>[2x]SNAMLVKLAVLFSGNGSNLENILEKLHKKTIGENTYEIVLCLCNKKDAFGIQRAKKFGLNTVIIDHKAYNTREEFDTIL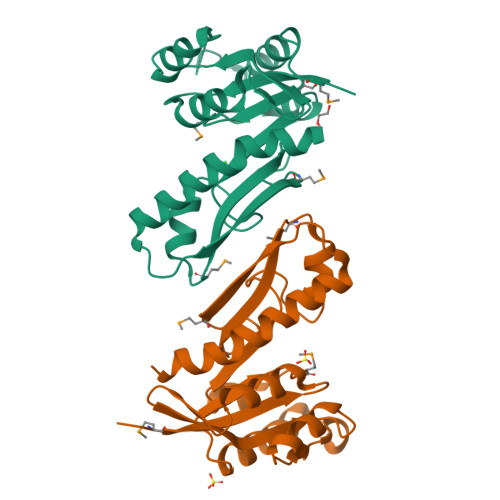VQKIKESGANLTVLAGFMRILSPVFTKNIKAINLHPSLLPLFKGAHAIKESYESDMKVAGVSVHWVSEELDGGMIIAQKAFEKRNLSFEEFEEKIHSLEHEILPLSVIEIFS>[2x]MRVLGIETSCDETAVAVLDDGKNVVVNFTVSQIEVHQKFGGVVPEVAARHHLKNLPILLKKAFEKVPPETVDVVAATYGPGLIGALLVGLSAAKGLAISLEKPFVGVNHVEAHVQAVFLANPDLKPPLVVLMVSGGHTQLMKVDEDYSMEVLGETLDDSAGEAFDKVARLLGLGYPGGPVIDRVAKKGDPEKYSFPRPMLDDDSYNFSFAGLKTSVLYFLQREKGYKVEDVAASFQKAVVDILVEKTFRLARNLGIRKIAFVGGVAANSMLREEVRKRAERWNYEVFFPPLELCTDNALMVAKAGYEKAKRGMFSPLSLNADPNLNV;>[2x]MGHHHHHHENLYFQGYNTVEEQKMRHLRFENLTEEQLKRLAKILTENLKGGEVVILSGNLGAGKTTFVKGMIRAIGLDEKMVKSPTFTLMNVYPGLKTIYHL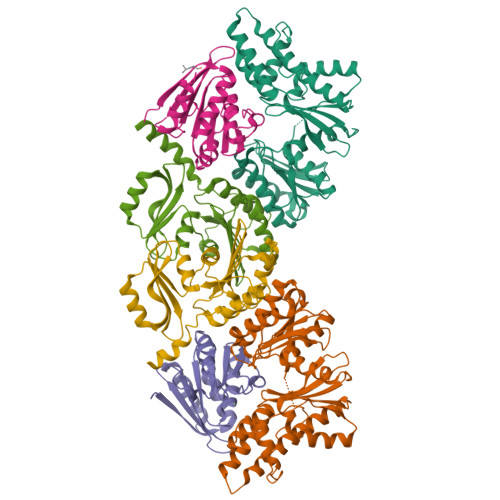DLYRLQDTDFLSLDVEDILEDEDGIMVVEWGDLFDGFWPEDSIKVKIEIADESHRNVEILIPEEVNFLVEKIERYRKELQNT;>MNVLALDTSQRIRIGLRKGEDLFEISYTGEKKHAEILPVVVKKLLDELDLKVKDLDVVGVGIGPGGLTGLRVGIATVVGLVSPYDIPVAPLNSFEMTAKSCPADGVVLVARRARKGYHYCAVYLKDKGLNPLKEPSVVSDEELEEITKEFSPKIVLKDDLLISPAVLVEESERLFREKKTIHYYEIEPLYLQKSIAELNWEKKKRG[2x]>[8x]SMADRGDSGDSDFVVVANRLPIDLERAPDGTTSWKRSPGGLVTALEPLLRRRRGAWIGWPGIPDSDEDPIVDGDLVLYPVRLSADDVAQYYEGFSNATLWPLYHDVIVKPIYNRQWWERYVEVNRRFAEATSRAAARGATVWVQDYQLQLVPKMLRELRPDLTIGFFLHIPFPPVELFMQLPWRTEITDGLLGADLVGFHLPGGAQNFLFLARRLVGANTSRASVGVRSKFGEVQIGSRTVKVGAFPISIDSADLDRQARQRSIRQRARQIRAELGNPRRILLGVDRLDYTKGIDVRLQAFAELLAEGRVNREDTVFVQLATPSRERVEAYRLLRDDIERQVGHINGEYGEVGHPVVHYLHRPVPREELIAFFVAADVMLVTPLRDGMNLVAKEYVACRSDLGGALVLSEFTGAAAELGQAYLVNPHNLDHVKDTMVAALNQTPEEGRRRMRALRRQVLAHDVDLWARSFLDALASTRTGDADAVPV

OtsA is a glycosyltransferase that uses the α anomer of G6P as acceptor and NDP-glucose as the donor to synthesize T6P. In this pathway, which is conserved and essential in mycobacteria, trehalose is synthesized in a two-step process involving OtsA and OtsB2 enzymes. MtrOtsA is composed of two Rossmann-fold domains with a deep catalytic site at their interface, in an arrangement typical of GT-B glycosyltransferases for other organisms. MtrOtsA forms a tetramer in solution, as previously observed for M. tuberculosis OtsA.

Although we did not observe any effect of F6P on enzyme activity for MtrOtsAs, we nevertheless attempted to soak this compound in both apo form and OtsA:ADP:G6P ternary complex crystals and also cocrystallize it in the presence and absence of ADP and G6P, all under CHES-free conditions. None of these conditions provided a structure in which F6P occupied an allosteric site. We could, however, observe F6P when cocrystallized together with ADP, bound to the acceptor substrate site, with OtsA presenting the active site in a closed conformation. The structure obtained with F6P shows this compound occupying the donor site, in the presence of ADP, with the enzyme adopting a closed conformation. Nevertheless, OtsA could use only G6P as an acceptor, and F6P showed no effect on the enzyme activity, indicating that the presence of F6P in the acceptor site was forced by the high concentration used for cocrystallization (5 mM).> MKSVKYISNMSKQEKGYRVYVNVVNEDTDKGFLFPSVPKEVIENDKIDELFNFEHHKPYVQKAKSRYDKNGIGYKIVQLDEGFQKFIEL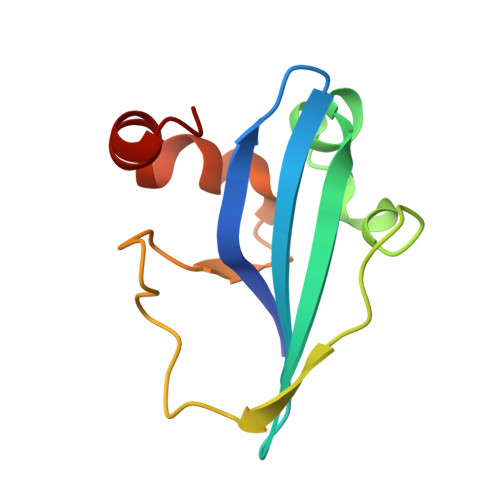NKEKMKENLDY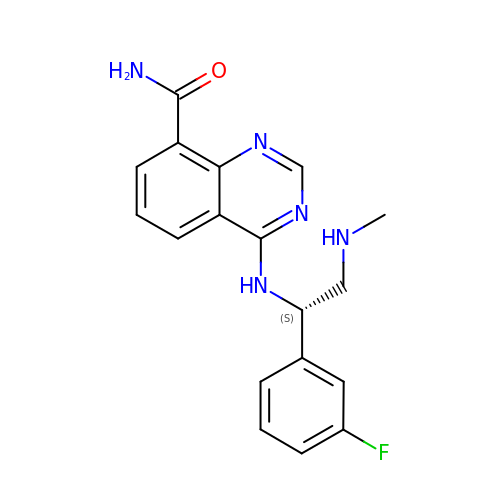4-{[(1S)-1-(3-fluorophenyl)-2-(methylamino)ethyl]amino}quinazoline-8-carboxamide | C18 H18 F N5 O | RBMOLIOJAWRTIV-OAHLLOKOSA-N> GMIQLQNPSHPTGLLCKANQMRLAGTL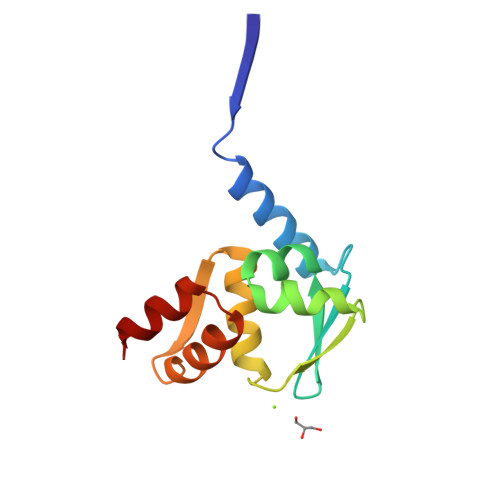CDVVIMVDSQEFHAHRTVLACTSKMFEILFHRNSQHYTLDFLSPKTFQQILEYAYTATLQAKAEDLDDLLYAAEILEIEYLEEQCLKML>[2x]MEFTTGLMSLDTALNEMLSRVTPLTAQETLPLVQCFGRILASDVVSPLDVPGFDNSAMDGYAVRLADIASGQPLPVAGKSFAGQPYHGEWPAGTCIRIMWGAPVPE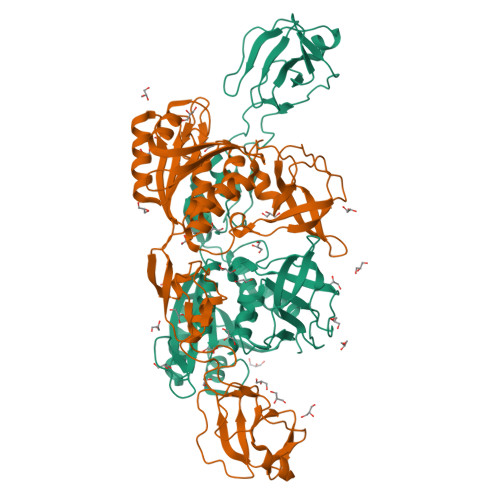GCEAVVMQEQTEQMDNGVRFTAEVRSGQNIRRRGEDISAGAVVFPAGTRLTTAELPVIASLGIAEVPVIRKVRVALFSTGDELQLPGQPLGDGQIYDTNRLAVHLMLEQLGCEVINLGIIRDDPHALRAAFIEADSQADVVISSGGVSVGEADYTKTILEELGEIAFWKLAIKPGKPFAFGKLSNSWFCGLPGNPVSATLTFYQLVQPLLAKLSGNTASGLPARQRVRTASRLKKTPGRLDFQRGVLQRNADGELEVTTTGHQGSHIFSSFSLGNCFIVLERDRGNVEVGEWVEVEPFNALFGGL Pf4 exists as a prophage in PAO1 and encodes a homologue of the P2 phage repressor C and was recently named Pf4r. X-ray crystal structure analysis shows that Pf4r forms symmetric homo-dimers homologous to the E.coli bacteriophage P2 RepC protein. Li et al. demonstrated that repressor C, which they named Pf4r, was responsible for immunity to Pf4 infection and also regulated replication of the Pf4 phage by repressing the expression of xisF4. Central to these effects of the Pf4 phage in P. aeruginosa is the repressor protein, Pf4r, which not only controls immunity to infection and phage replication but also acts to regulate the expression of host genes.

The mutated Pf4r, with non-synonymous mutations, will be referred to here as Pf4r*. However, we were successful in generating high-quality crystals for the Pf4r* mutant from which the structure was directly determined and from which the Pf4r structure was modelled. The Pf4r* structure was solved initially by single anomalous dispersion (SAD) and then by molecular replacement (MR) to a final resolution of 1.97 Å in the space group C 2 2 21, yielding an asymmetric unit containing two protein chains (A and B). An Arg to Leu substitution at position 80 (blue spheres) maps to an exposed surface of the protein on the opposite side of the dimer complex from the predicted DNA-binding motif and also well away from the dimerisation interface. We do not predict this mutation to affect DNA binding or dimerisation, but it is possible it may affect some protein–protein interaction with a currently unknown partner. The second mutation, a Ser to Pro mutation at residue 4 (78879A>G), was observed to reside directly at the dimer interface (pink spheres). The mutation in Pf4r* to proline at position 4 may mean that only weaker hydrophobic interactions can be made, and the homodimerisation may be less stable. In contrast, Pf4r* eluted as a monomer with a molecular mass equivalent of a dimer as determined by MALS. This would suggest that the mutations in Pf4r* significantly reduce dimerisation and hence, prevent DNA binding.

>[2x]MSTPADRARLLIKKIGPKKVSLHGGDYERWKSVSKGAIRVSTEEIDVLVKIFPNYALWIASGSIAPEVGQTSPDYDEANLNLSNQNAGAHHHHHH SULFUR OXIDE | O S | 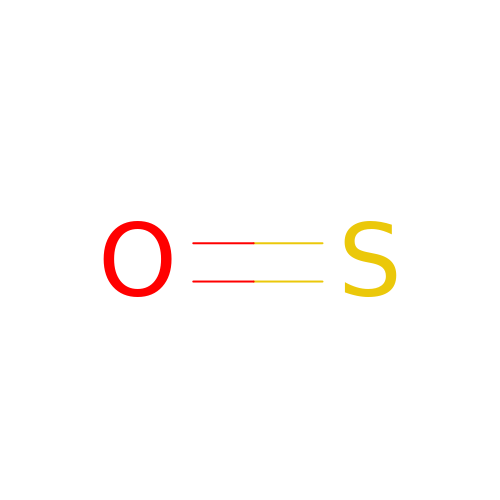XTQHKBHJIVJGKJ-UHFFFAOYSA-N6-{[3-chloro-4-(4-methylpiperazin-1-yl)phenyl]amino}-1-[6-(2-hydroxypropan-2-yl)pyridin-2-yl]-2-(prop-2-en-1-yl)-1,2-dihydro-3H-pyrazolo[3,4-d]pyrimidin-3-one 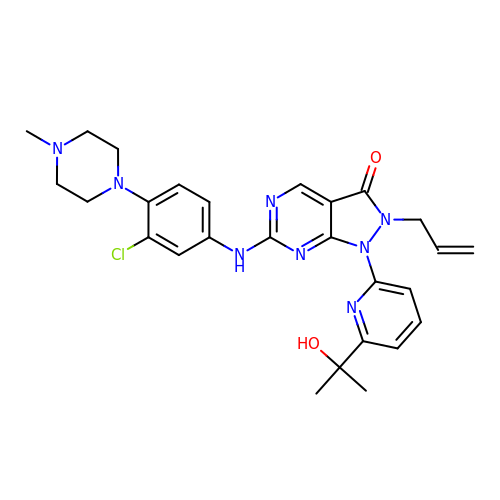| C27 H31 Cl N8 O2 | ILJROYVRHXGGKS-UHFFFAOYSA-N>[2x]MAGSGAWKRLKSMLRKDDAPLFLNDTSAFDFSDEAGDEGLSRFNKLRVVVADDGSE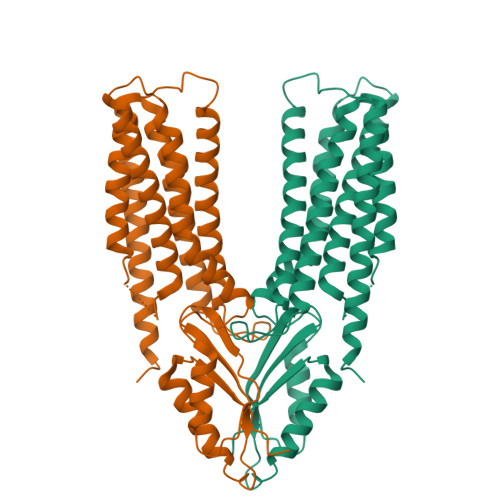APERPVNGAHPTLQADDDSLLDQDLPLTNSQLSLKVDSCDNCSKQREILKQRKVKARLTIAAVLYLLFMIGELVGGYIANSLAIMTDALHMLTNLSAIILTLLALWLSSKSPTKRFTFGFHRLEVLSAMISVLLVYILMGFLLYEAVQRTIHMNYEINGDIMLITAAVGVAVNVIMGFLLNQSGHRHSHSHSLPSNSPTRGSGCERNHGQDSLAVRAAFVHALGNLVQSVGVLIAAYIIRFKPEYKIADPICTYVFSLLVAFTTFRIIWDTVVIILEGVPSHLNVDYIKEALMKIEDVYSVEDLNIWSLTSGKSTAIVHIQLIPGSSSKWEEVQSKANHLLLNTFGMYRCTIQLQSYRQEVDRTCANCQSSSPGSIEGRIVKDYKDDDDK>MELVVKSVAAASVKTATLVIPVGENRKLGAVAKAVDLASEGAISAVLKRGDLAGKPGQTLLLQNLQGLKAERVLLVGSGKDEALGDRTWRKLVASVAGVLKGLNGADAVLALDDVAVNNRDAHYGKYRLLAETLLDGEYVFDRFKSQKVEPRALKKVTLLADKAGQAEVERAVKHASAIATGMAFTRDLGNLPPNLCHPSFLAEQAKELGKAHKALKVEVLDEKKIKDLGMGAFYAVGQGSDQPPRLIVLNYQGGKKADKPFVLVGKGITFDTGGISLKPGAGMDEMKYDMCGAASVFGTLRAVLELQLPVNLVCLLACAENMPSGGATRPGDIVTTMSGQTVEILNTDAEGRLVLCDTLTYAERFKPQAVIDIATLTGACIVALGSHTTGLMGNNDDLVGQLLDAGKRADDRAWQLPLFDEYQEQLDSPFADMGNIGGPKAGTITAGCFLSRFAKAYNWAHMDIAGTAWISGGKDKGATGRPVPL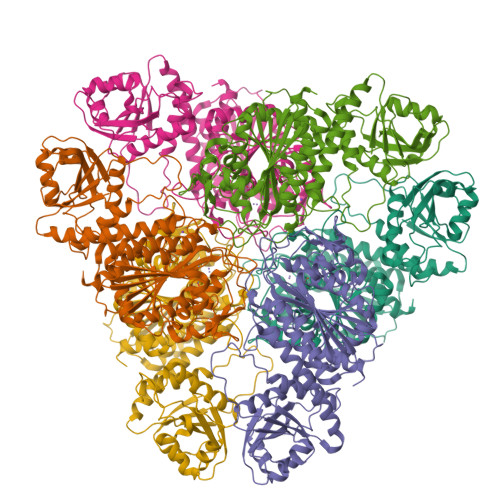LTQYLLDRAGA[6x]> KLCSLDNGDCDQFCHEEQNSVVCSCARGYTLA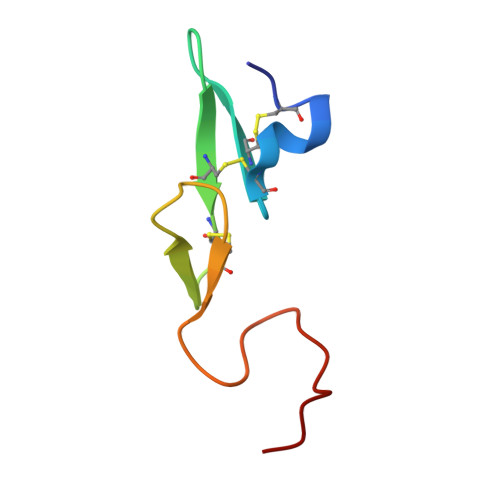DNGKACIPTGPYPCGKQTLERR2-[[(2~{S})-2,3-bis(oxidanyl)propyl]-[2-(6-oxidanylidene-1~{H}-purin-9-yl)ethyl]amino]ethylphosphonic acid | C12 H20 N5 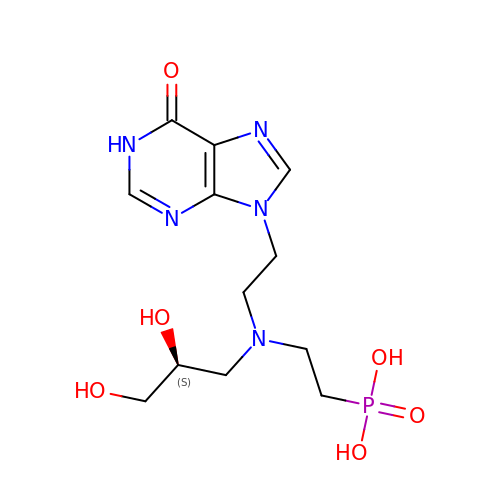O6 P | XBILBXZMSMIUBY-VIFPVBQESA-N>MLFHVKMTVKLPVDMDPAKATQLKADEKELAQRLQREGTWRHLWRIAGHYANYSVFDVPSVEALHDTLMQLPLFPYMD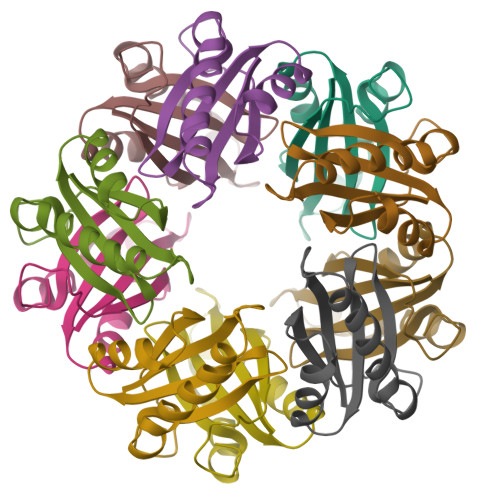IEVDGLCRHPSSIHSDDR[10x]> GPEFGSTNMASRYEKEFLEVEKIGVGEFGTVYKCIKRLDGCVYAIKRSMKTFTELSNENSALHEVYAHAVLGHHPHVVRYYSSWAEDDHMIIQNEYCNGGSLQAAISENTKSGNHFEEPKLKDILLQISLGLNYIHNSSMVHLDIKPSNIFICHKMQSESSGVIEEVENEADWFLSANVMYKIGDLGHATSINKPKVEEGDSRFLANEILQEDYRHLPKADIFALGLTIAV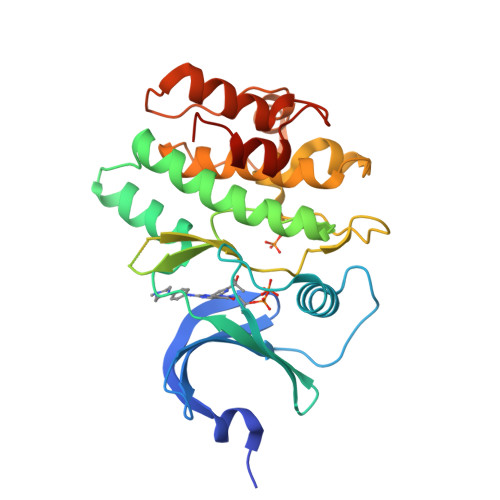AAGAESLPTNGAAWHHIRKGNFPDVPQELSESFSSLLKNMIQPDAEQRPSAAALARNTVLRPSLGK>[5x]QEEGEDNGGEDNKKLRGALSSAILSEKPNVKWEDVAGLEGAKEALKEAVILPVKFPHLFKGNRKPTSGILLYGPPGTGKSYLAKAVATEANSTFFSVSSSDLVSKWMGESEKLVKQLFAMARENKPSIIFIDEVDALTGTRGEGESEASRRIKTELLVQMNGVGNDSQGVLVLGATNIPWQLDSAIRRRFERRIYIPLPDLAARTTMFEINVGDTPCVLTKEDYRTLGAMTEGYSGSDIAVVVKDALMQPIRKIQSATHFKDVSTEDDETRKLTPCSPGDDGAIEMSWTDIEADELKEPDLTIKDFLKAIKSTRPTVNEDDLLKQEQFTRDFGQEGN;> XDEIVNKVLX

The Endosomal Sorting Complexes Required for Transport (ESCRT) pathway drives multiple cellular membrane fission processes through the formation of filaments comprising different subsets of related ESCRT-III family members. ESCRT-III filaments stabilize highly curved membrane necks that resolve by fission when the filaments are remodeled by Vps4. Vps4 is monomeric or dimeric at cytoplasmic concentrations, but forms a hexamer when active and recruited to ESCRT-III filaments. The Vps4 N-terminal MIT domain is followed by an ~40 residue flexible linker and an ATPase cassette that comprises a large ATPase domain, small ATPase domain, and a β domain.

We have now determined the Vps4-ESCRT-IIIpeptide complex structure at 3.2 Å resolution. Vps4 subunits A-E form a helix whose symmetry approximates a 60° rotation and 6.3 Å translation between adjacent subunits, and provides the binding surface for the ESCRT-III peptide. The peptide adopts an extended conformation that resembles a canonical β-strand (phi −92° to −151°; psi 102° to 189° (−171°)) and packs closely against Vps4 subunits A-E. Two distinct classes of side chain binding sites propagate along the pore. Odd-numbered ESCRT-III residues (D1, I3, N5, V7) bind in ‘class I’ pockets, while the side chains of even-numbered ESCRT-III residues (E2, V4, K6, L8) bind in ‘class II’ pockets. Class I pockets are formed by pore loop 1 residues K205 and W206, with substrate side chains sandwiched between W206 from successive subunits. The class II pockets are formed by the pore loop 1 M207 residues of successive subunits, and are flanked by pore loop 2 residues of the first Vps4 subunit and, to a greater extent, by the pore loop 2 residues of the preceding subunit. The refined model indicates that the NH groups of the even-numbered ESCRT-III peptide residues form hydrogen bonds with the main chain O of Vps4 K205 (subunit A, B, C, and D distances are 3.1–3.5 Å). Nucleotides primarily contact one Vps4 subunit at a subunit interface, with the β-phosphate and BeFx contacting two ‘finger’ arginines, R288 and R289, from the following subunit. The bound ADP·BeFx mimics ATP binding to subunits A, B, and C, whereas subunits D and E appear to bind ADP.>MVRDMKH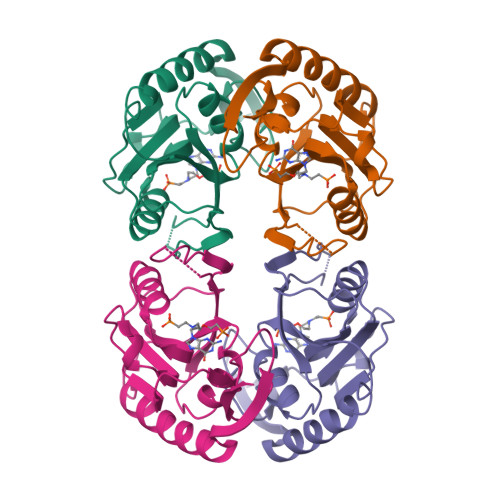TVEVMIPEAEIKARIAELGRQITERYKDSGSDMVLVGLLRGSFMFMADLCREVQVSHEVDFMTASSYGSGMSTTRDVKILKDLDEDIRGKDVLIVEDIIDSGNTLSKVREILSLREPKSLAICTLLDKPSRREVNVPVEFIGFSIPDEFVVGYGIDYAQRYRHLPYIGKVILLDE[2x]>[5x]MHHHHHHTPTAQTTASARRVVFPFTAIVGQEEMKLALLLNVIDPKIGGVMIMGDRGTG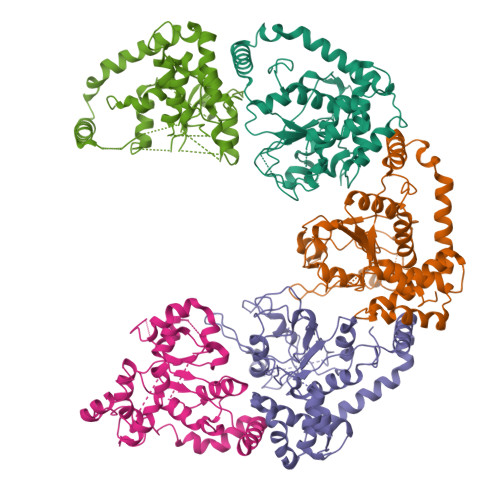KSTTIRALADLLPEIPVVANDPFNSDPSDPDLMSDEVRQKSGTGAEIPIEFKKVQMVDLPLGATEDRVCGTIDIEKALSEGVKAFEPGLLAKANRGILYVDEVNLLDDHLVDVLLDSAASGWNTVEREGISIRHPARFVLVGSGNPEEGELRPQLLDRFGMHAEIHTVKEPALRVQIVEQRSEFDQNPPTFLEKYNPEQTALQKKIVEAQKLLPEVKLDYDLRVKISEVCSELDVDGLRGDIVTNRAAKALTAYEGRTEVTVDDIRRVITLCLRHRLRKDPLESIDSGYKVEKVFARIFGVELLEDDSSQKNGAGQIKTGVR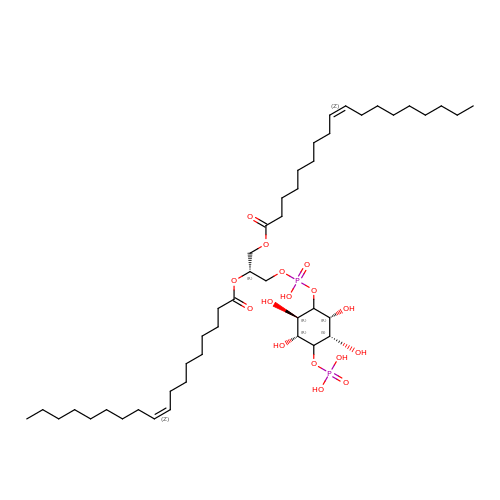(2R)-3-{[(S)-hydroxy{[(1R,2R,3R,4R,5S,6R)-2,3,5,6-tetrahydroxy-4-(phosphonooxy)cyclohexyl]oxy}phosphoryl]oxy}propane-1,2-diyl di[(9Z)-octadec-9-enoate] | C45 H84 O16 P2 | XIBQVFRCUJZPTP-NHVDGIRCSA-N> MESLPVIAAPSMWTRPQIKDFKEKIQQDADSVITVGRGEVVTVRVPTHEEGSYLFWEFATDNYDIGFGVYFEWTDSPNTAVSVHVSESSDDDEEEEENIGCEEKAKKNANKPLLDEIVPVYRRDCHE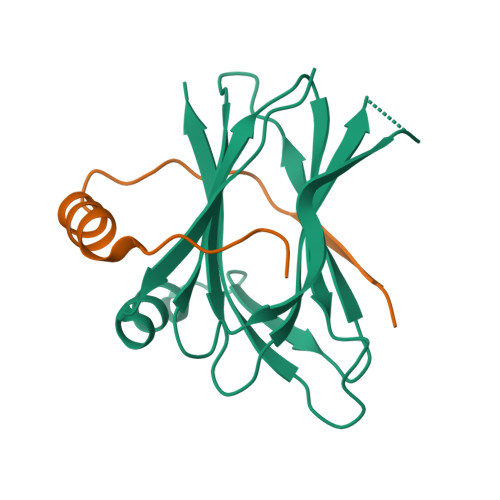EVYAGSHQYPGRGVYLLKFDNSYSLWRSKSVYYRVYYTR;> GNRVIDAEPREIPLEYADDLLEAMAHHRPVPCSLGLSQAIANNTPIQQISETFWKYRK> GHMSRLEIYSPEGLRLDGRRWNELRRFESSINTHPHAADGSSYMEQGNNKII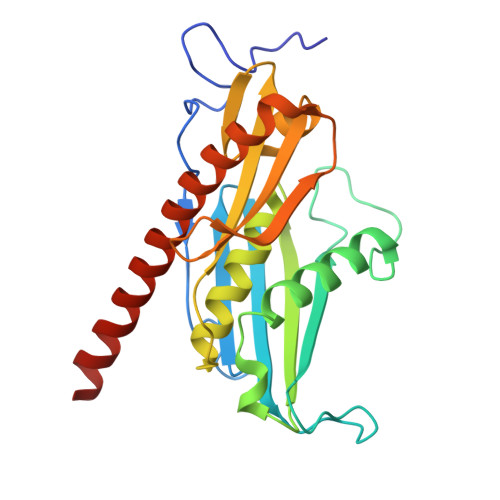TLVKGPKEPRLKSQMDTSKALLNVSVNITKFSKFERSKSSHKNERRVLEIQTSLVRMFEKNVMLNIYPRTVIDIEIHVLEQDGGIMGSLINGITLALIDAGISMFDYISGISVGLYDTTPLLDTNSLEENAMSTVTLGVVGKSEKLSLLLVEDKIPLDRLENVLAIGIAGAHRVRDLMDEELRKHAQKRVSNASAR> HHHHHHENLYFQGEETDTKIYFDASNLPAEWGTTKTVYCHLYAVAGDDLPETSWQGKAEKCKKDTATGLYYFDTAKLKSADGTNHGGLKDNADYAVIFSTIDTKSQSHQTCNVTLGKPCLGDTIYLTGGTVENTEDSSKRDFAAT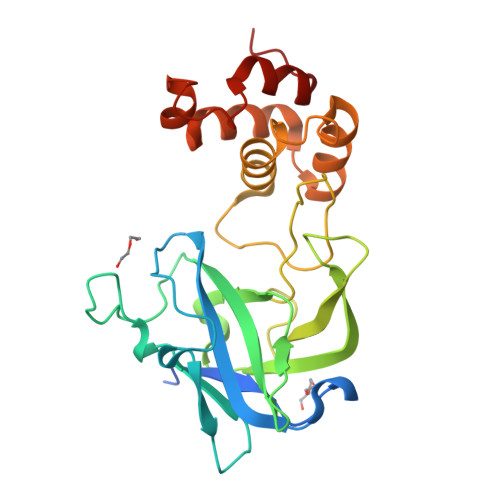WKNNSDNYGPKAAITSLGHVTEGRFPIYLSRAEMVAQAIFNWAVKNPKNYTPETVADICAQVEAEPMDVYNAYAEMYATELADPAAYPDCAPLTTVATLLGVDPSG(2R,3R)-3-methyl-4-(2-oxidanylidene-2-propan-2-yloxy-ethyl)sulfanyl-2-[(2R)-3-oxidanyl-1-oxidanylidene-butan-2-yl]-2,3-dihydro-1H-pyrrole-5-carboxylic acid | C15 H23 N O6 S | 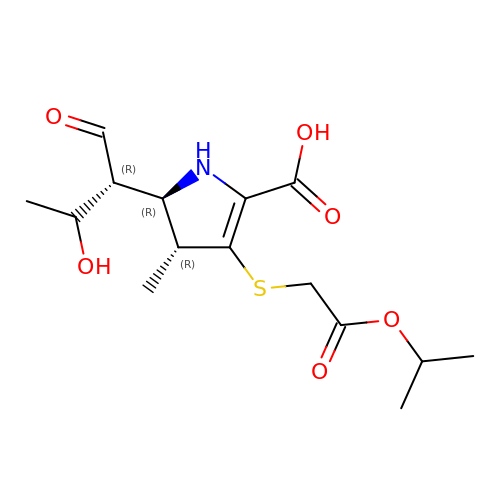BCFABNCZHGBALS-QARRAHMOSA-N>[4x]GSPSR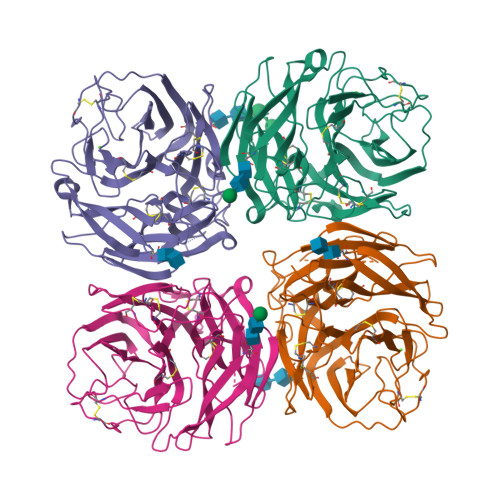ATPLVLGENLCSINGWVPTYRGEGTTGKIPDEQMLTRQNFVSCSDKECRRFFVSMGYGTTTNFADLIVSEQMNVYSVKLGDPPTPDKLKFEAVGWSASSCHDGFQWTVLSVAGDGFVSILYGGIITDTIHPTNGGPLRTQASSCICNDGTCYTIIADGTTYTASSHRLYRLVNGTSAGWKALDTTGFNFEFPTCYYTSGKVKCTGTNLWNDAKRPFLEFDQSFTYTFKEPCLGFLGDTPRGIDTTNYCDKTTTEGEGGIQGFMIEGSNSWIGRIINPGSKKGFEIYKFLGTLFSVQTVGNRNYQLLSNSTIGRSGLYQPAYESRDCQELCFWIEIAATTKAGLSSNDLITFCGTGGSMPDVNWG(2R)-({N-[(3S)-3-({[(3S,6S)-6-CYCLOHEXYL-5,8-DIOXO-4,7-DIAZABICYCLO[14.3.1]ICOSA-1(20),16,18-TRIEN-3-YL]CARBONYL}AMINO)-2-OXOHEXANOYL]GLYCYL}AMINO)(PHENYL)ACETIC 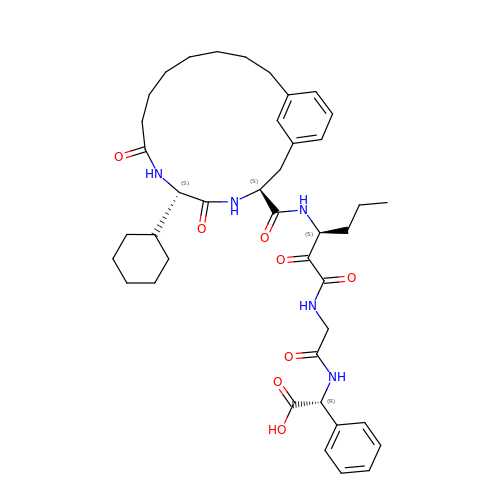ACID | C41 H55 N5 O8 | MRGBFMHIJSOQIX-IMJQVECRSA-N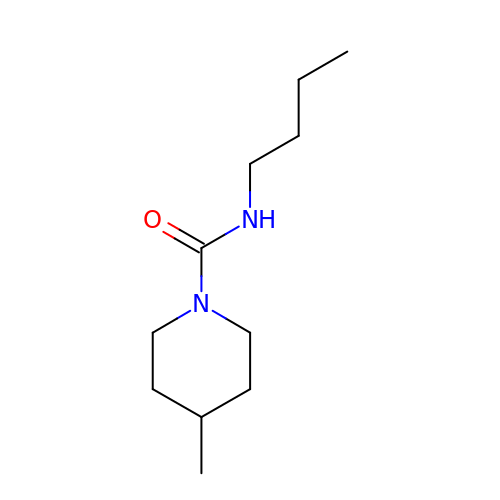~{N}-butyl-4-methyl-piperidine-1-carboxamide | C11 H22 N2 O | GASMLRFTKRLWLW-UHFFFAOYSA-N>[5x]MDSGDGQDLRAFVHDSPEETETTQRLTKLLTNSPIPTEELVNNLPLFLRRHQMTDLLSMDALYRQVLDVPGVIMEFGVRFGRHLGTFAALRGVYEPYNPLRRIVGFDTFTGFPDVNDVDRVGPTAYQGRFAVPGGYPAYLKEVLDAHECSDFFGHVTQRSVLVEGDVRETVPRYLAENPQTVIALAYFDLDLYEPTKAVLEAIRPYLTKGSIVAFDELDNPKWPGENIAMRKVLGLDHAPLRLLPGRPAPAYLRWGD

CalS11 uses S-adenosylmethionine (AdoMet, SAM) as the methyl donor. Structural flexibility and dynamics are generally key for protein function. The sequence identity of NovP and CalS11 is 20%.

The general fold of CalS11 is stable in structures with or without SAH bound. Superimposition of apo (red) and complexed (blue) CalS11 structures. residues 111–131 are missing in the electron density. of CalS11 shows enhanced mobility in the absence of substrate. binding site is more solvent accessible when no substrate is bound. completely exposed to solvent in many conformations. distributed between closed and open states.The bacteriophage ϕ29, a representative of bacteriophages with a short non-contractile tail, has an ~19 kb dsDNA genome encoding ~20 proteins. Both 5ʹ ends of the genome are covalently connected to the terminal protein gene product 3 (gp3). ϕ29 infects the Gram-positive Bacillus subtilis cells by injecting the genome–gp3 complex into the host-cell cytoplasm using a short non-contractile tail, leaving the genome emptied virion on the cell surface. Here, we report the cryo-electron microscopy (cryo-EM) structural studies of the ϕ29 prohead, the mature and the genome-emptied virions at near-atomic resolutions up to 3.2 Å. Our results show structural details of the complex capsid, the DNA packaging motor and the entire tail machinery, and provide a molecular basis for understanding the assembly, maturation and infection mechanisms of the bacteriophage ϕ29.

We calculated the cryo-electron microscopy (cryoEM) reconstructions of the ϕ29 prohead, the mature head and the genome emptied head to a resolution of 3.6, 3.2, and 3.2 Å, respectively. Our results showed that the 448-amino-acid-long polypeptide chain of the major capsid protein gp8 folds into three structural domains: the small N-terminal helix domain (the gp8-N-helix domain, residues 1–61), the central HK97 fold domain (the gp8-HK97 domain, residues 62–347) and the C-terminal immunoglobulin-like domain (the gp8-C-Ig domain, residues 348–448). The total 235 gp8 subunits assemble into a ~520 Å long and 400 Å wide, T = 3, Q = 5 prolate icosahedron of 30 flat hexameric capsomeres and 11 concave pentameric capsomeres. Structural comparisons using the HK97 domains showed significantly greater variation in the hexameric capsomeres than that in the pentameric capsomeres (an average r.m.s.d. of 2.2 Å vs. 0.6 Å between the aligned Cα atoms of the corresponding HK97 domains of the mature head capsomeres). With the cryoEM map of the mature head calculated at a resolution of 3.2 Å, we determined the structure of the pseudo-hexagonal base of the head fiber (residues 1–110 of gp8.5). Six β-barrel domains from three gp8.5 monomers form the pseudo-hexagonal base of each head fiber, which interact with one C-Ig from a pentameric capsomer with a contact surface area of ~620 Å2 and two C-Igs each from a different hexameric capsomer with an average contact surface area of ~400 Å2. Further analysis showed that the icosahedral end caps of the mature head expanded slightly upon the loading of the genome. However, structural comparisons of individual hexameric and pentameric capsomeres within the icosahedral end caps showed a similar average r.m.s.d. of 0.4 Å, indicating that the expansion in the icosahedral end caps mainly occurs through the rigid-body movements of the capsomeres. As have been shown in the head comparisons, the E loop in contact with the pRNA has an outward shift of ~3 Å in the mature head. In addition, we did not observe any pRNA density in the 3.2 Å mature capsid map.

>[235x]MRITFNDVKTSLGITESYDIVNAIRNSQGDNFKSYVPLATANNVAEVGAGILINQTVQNDFITSLVDRIGLVVIRQVSLNNPLKKFKKGQIPLGRTIEEIYTDITKEKQYDAEEAEQKVFEREMPNVKTLFHERNRQGFYHQTIQDDSLKTAFVSWGNFESFVSSIINAIYNSAEVDEYEYMKLLVDNYYSKGLFTTVKIDEPTSSTGALTEFVKKMRATARKLTLPQGSRDWNSMAVRTRSYMEDLHLIIDADLEAELDVDVLAKAFNMNRTDFLGNVTVIDGFASTGLEAVLVDKDWFMVYDNLHKMETVRNPRGLYWNYYYHVWQTLSVSRFANAVAFVSGDVPAVTQVIVSPNIAAVKQGGQQQFTAYVRATNAKDHKVVWSVEGGSTGTAITGDGLLSVSGNEDNQLTVKATVDIGTEDKPKLVVGEAVVSIRPNNASGGAQA;>[165x]MMVSFTARAKSNVMAYRLLAYSQGDDIIEISHAAENTIPDYVAVKDVDKGDLTQVNMYPLAAWQVIAGSDIKVGDNLTTGKDGTAVPTDDPSTVFGYAVEEAQEGQLVTLVISRSKEISIEVEDIKDAGDTGKRLLKINTPSGARNIIIENEDAKALINGETTNTNKKNLQDLLFSDGNVKAFLQATTTDENKTALQQLLVSNADVLGLLSGNPTSDNKINLRTMIGAGVPYSLPAATTTTLGGVKKGAAVTASTATDVATAVKDLNSLITVLKNAGIISL> MSRSAYEDDIR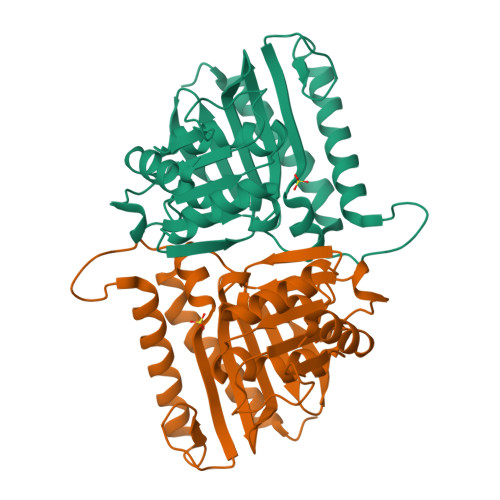LAHRLADVAADIIRPFFRAPLTIDLKADHSPVTKADRGAEQAMRAILEQERPEDGIFGEEMGVSRPDARRLWVLDPIDGTRAFIGGRASFGTLIALVEDGRPVLGIINQPIHQERWVGVKDLPTSFNGEVIHTRSCPALDHALLATTSPWLFEKEGEVHFDKIRLKCRDTLLGGDCYNYGLLSLGHCDLVVEQGLKFYDFAALVPIVEGAGGIMRDWQNRPLNKNSVGEVIAAGDHHLIEPALSAMEL> MFLPPPECPVFEPSWEEFADPFAFIHKIRPIAEQTGICKVRPPPDWQPPFACDVDKLHF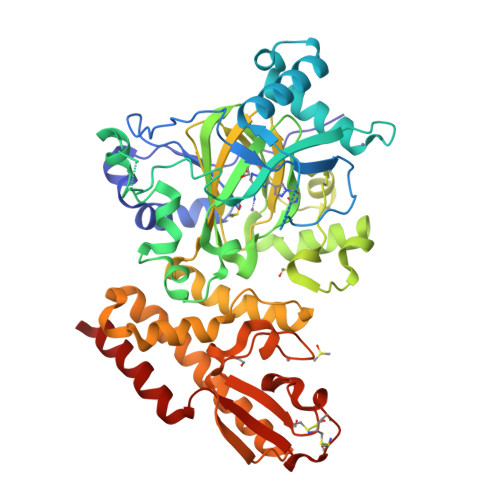TPRIQRLNELEAQTRVKGGGGARDYTLRTFGEMADAFKSDYFNMPVHMVPTELVEKEFWRLVSTIEEDVTVEYGADIASKEFGSGFPVRDGKIKLSPEEEEYLDSGWNLNNMPVMEQSVLAHITADICGMKLPWLYVGMCFSSFCWHIEDHWSYSINYLHWGEPKTWYGVPGYAAEQLENVMKKLAPELFVSQPDLLHQLVTIMNPNTLMTHEVPVYRTNQCAGEFVITFPRAYHSGFNQGFNFAEAVNFCTVDWLPLGRQCVEHYRLLHRYCVFSHDEMICKMASKADVLDVVVASTVQKDMAIMIEDEKALRETVRKLGVIDSERMDFELLPDDERQCVKCKTTCFMSAISCSCKPGLLVCLHHVKELCSCPPYKYKLRYRYTLDDLYPMMNALKLRAES>[8x]GGPMDASVEEEGVRRALDFAVGEYNKASNDMYHSRALQVVRARKQIVAG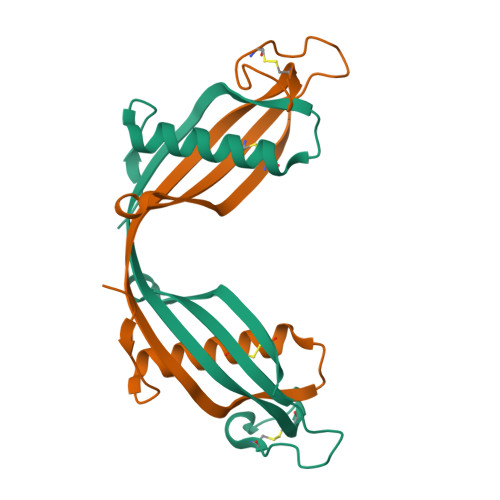VNYFLDVELGRTTCTKTQPNLDNCPFHDQPHLKRKAFCSFQIYAVPWQGTMTLSKSTCQDA> MELWLVRHGETLWNREGRLLGWTDLPLTAEGEAQARRLKGALPSLPAFSSDLLRARRTAELAGFSPRLYPELREIHFGALEGALWETLDPRYKEALLRFQGFHPPGGESLSAFQERVFRFLEGLKAPAVLFTHG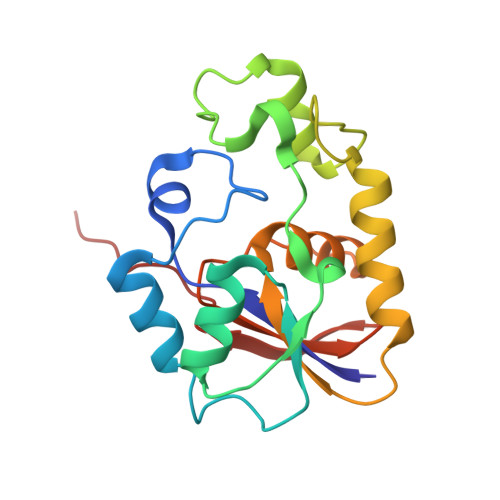GVVRAVLRALGEDGLVPPGSAVAVDWPRRVLVRLAMDGEEATG Pur-α is a ubiquitous, highly conserved protein involved in a variety of cellular processes such as transcription, cell cycle control, mRNA transport, and neuronal development. This sequence repeat-containing protein binds specifically to RNA as well as to DNA and prefers the consensus sequence (GGN)n, where N is not guanine. When searching databases for proteins with PUR repeats in lower species, we found that a bacterial hypothetical protein (Borrelia burgdorferi B31 gene bank entry BB0047) contains a single PUR repeat. We found that the B. burgdorferi Pur-α and the nucleic acid-binding region of human Pur-α bound with comparable affinities to DNA oligomers with (GGN)n sequences.

Crystals of selenomethione-substituted B. burgdorferi Pur-α 8–105 (L17M, F27M, I64M) belonged to space group I212121 and diffracted up to 1.9 Å resolution. The PUR repeat of B. burgdorferi Pur-α crystallized as a strongly intertwined dimer. Each PUR repeat is comprised of a four-stranded anti-parallel β-sheet followed by an α-helix. The interaction of two monomers results in a globular domain that we refer to as PUR domain. It exposes both α-helices on one side and both β-sheets on the opposing side. The buried surface interface reveals a large number of aliphatic and aromatic residues. The buried surface interface of 2058 Å2 significantly exceeds those observed for average crystal packing and strongly suggests the dimer is also stable in solution. The part of the crystallized protein that is visible in the experimental electron density (amino acids 8 to 84) matches the homology region that was identified as PUR repeat (amino acids 8 to 81). Thus, the structure confirms that a PUR repeat identified on the sequence level indeed corresponds to a structural entity. In the B. burgdorferi case, the interaction relies on a dimer built by two identical monomers, whereas in D. melanogaster Pur-α, an intra-molecular dimer is formed by its PUR repeats I and II.

>ERGEVYSEKMFTESERTYFMNVKENRKGDYFLNIVESKRSPSGDFERHSIFVYEENMNEFESNLLKAIAVIKQKVSTGSVGSSARHNKGYGEYGERSK[2x]>DYKDDDDKLHSQANLMRLKSDLFNRSPMYPGPTKDDPLTVTLGFTLQDIVKADSSTNEVDLVYYEQQRWKLNSLMWDPNEYGNITDFRTSAADIWTPDITAYSSTRPVQVLSPQIAVVTHDGSVMFIPAQRLSFMCDPTGVDSEEGATCAVKFGSWVYSGFEIDLKTDTDQVDLSSYYASSKYEILSATQTRQVQHYSCCPEPYIDVNLVVKFRERR[5x]

The soluble ACh-binding proteins (AChBP) from mollusks form homopentameric assemblies of subunits homologous to the N-terminal, extracellular ligand binding domain (LBD) of the nAChR (Figure A1). The binding pocket of AChBP possesses all of the functional residues identified in the nAChR LBD, and its extension toward various directions of the interface provides multiple means for selective accommodation of the nicotinic ligands. The ligand binding pocket encompasses a nest of five electron-rich aromatic side chains provided by residues Tyr93, Trp147, Tyr188 and Tyr195 on the principal (+) face of the subunit interface and residue Tyr55 on the complementary (−) face. This pocket is partially sheltered from the solvent by loop C, which is found at the outer perimeter of the pentamer and harbors at its tip a disulfide bridge linking the vicinal Cys190 and Cys191 residues, linked into a Cys-trans-Cys disulfide bridge (aka oxidized cysteinyl-cysteinyl ring), a signature determinant for nAChR α subunits.

The structures of A-AChBP bound with spiroimines (+)-4 R and (−)-4 S were solved in the 1.85–2.00 Å resolution range from preformed stoichiometric complexes. Despite the moderate binding affinities, the well-defined electron densities revealed full ligand occupancy at all five binding sites due to the high protein concentration (ca. 100-fold the Kd values) and slight molar excess of spiroimine over A-AChBP used for complex formation and crystallization (see Experimental procedures). Enantiomer (+)-4 R was a tighter binder to A-AChBP, albeit with a modest stereospecificity of up to two-fold arising largely from slower complex dissociation (lower koff values). As a result, the position of the cyclohexane ring is displaced toward the tip of loop C, and the dioxolane ring projects in the opposite direction at the entrance of the binding pocket, thus making limited interactions with the A-AChBP residues. Such a drastic shift in the position of the 3-ring system for the two enantiomers is associated with differences in the loop-C position (and see below) and may account for the slightly (ca. 2-fold) higher affinity of enantiomer (+)-4 R for the two AChBPs compared to enantiomer (−)-4 S. The smaller mean score for the interaction of enantiomer (+)-4 R at all five A-AChBP subunit interfaces compared to that for enantiomer (−)-4 S suggests tighter binding to A-AChBP, independently of the loop-C conformation. The ratio of the (+)-4 R/(−)-4 S mean scores, equal to 1.22, also indicates computational prediction from the structures for a tighter binding of enantiomer (+)-4 R, which should be reflected by a ca. one order of magnitude difference in the Kd values for the two complexes.> EIGEPDVTDATLGSVYSEIISPVKDCILTVA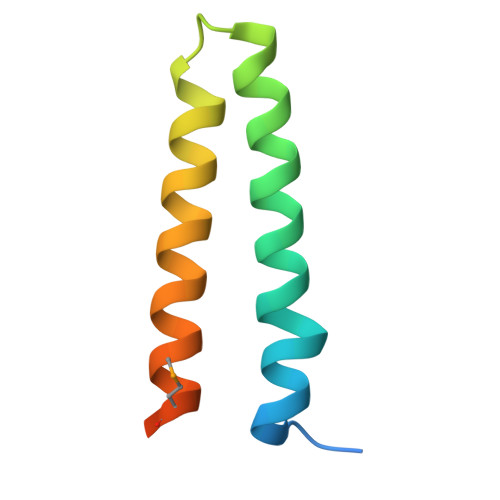KAVSFNPGGKDNTDAVEVLTELNTKVERAAMNQPILTTKTER> AMDKSAKAPQITIFDHRGCSRAPK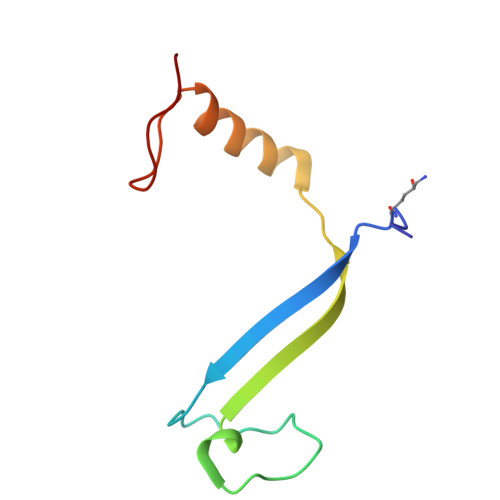ESTGGKAGGQDDEMMVKVASTKVTVSESDAAKKLQEFITFEKGIDGPFTSKN> MRPRRRGLAYHHTKPKGQLSQGHYPTTSNDGQRRKVGNSEAFQSFDIWKNLDRIRSTKKNAGQFIKGSLLILPMRTEDKQQFDECMDELHKYISKDILRCYPQKEQKDEGMLFYIVLKDFNILDSCFVLSVLLAFQKRLWMAPSEKSYFRVPKNINLTGSFYLPKNIETGRGHIITSYRREQPSSSIVEVGFNVVPDFQQFQVKACHVSKFMNELSNFFSQVEFGKCEANVINYFKREYNRTYSQISLALYELPLIGDGLFDIKSYISKTRP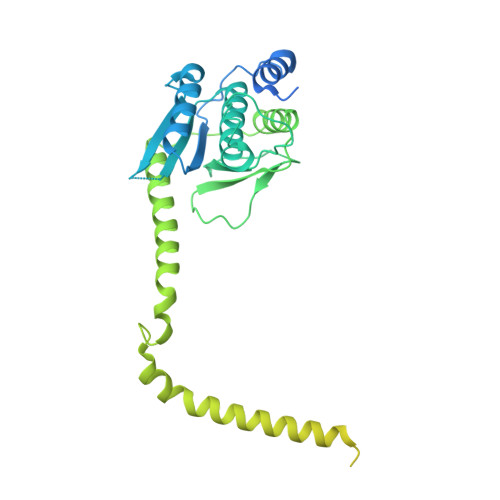IIETSKAQMIKHISEMKAYNEISGLQGDQFPRQQRPLSNSPSSNSISSSQTIEAGATSYQTQPQRHAVNKPSNVLNSSNRHSGPKTFEDGRYSEGNKPGFMTQDEIKQHCIGTIKASMDAVKKKSSYQILKTYVRCPRQNYIDIVYQNLNDLRSKTNCNIVVLNLNNLHESQMWLESLNTTNYTIFAQAPHPSTIRVISIGGVGEYIVKALELILNILEH> VNIVDYSDCFEGISGGAIFCNTKNKEYNIYNKELIETRRSPCSTFKIVSTLIGLEKGVINSKESVMGYDGTDYPNKNWNKNLSLEEAFKESCVWYYKKLINKVDAKSVQNI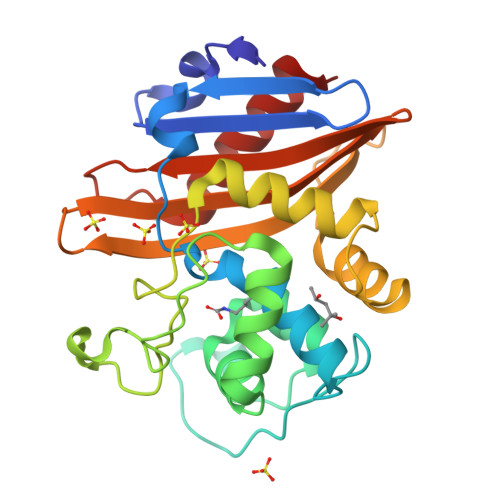LDDLKYGNCDISEWEGDLKNGKGHLNGFWLESSLQISPKEQVQTMAKIFEGDTNFKKEHINILRDIMAIDVNDANINVYGKTGTGFDEKNKRVDAWFVGMLEREGDTYYFAIKSDDSNKEITGPKVKEIAINIIKKYYS6-amino-2-({2-[4-(2-hydroxyethyl)phenyl]ethyl}amino)-1,7-dihydro-8H-imidazo[4,5-g]quinazolin-8-one | C19 H20 N6 O2 | 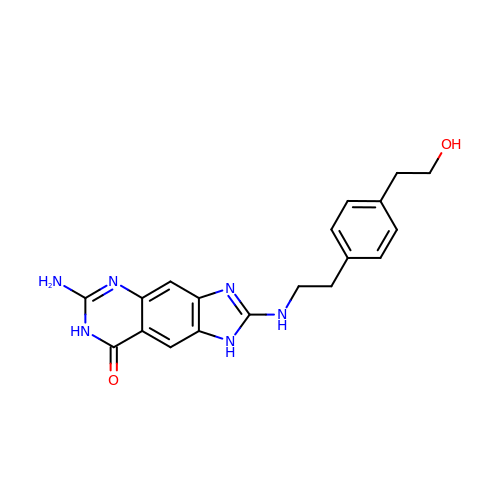RGCYFFRYXJGABS-UHFFFAOYSA-N>[5x]ARVNAQTGAPDILTSLDEKSVSYDTVMDKYWLSQYVIARETYDWYTLQKDYETVGMLSSPSEGQSYASQFQGD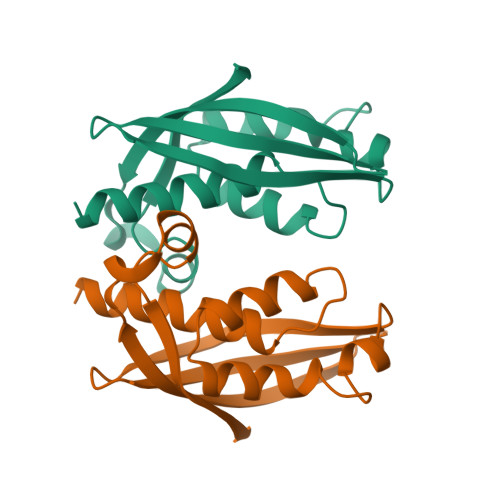KALDKQYGSNVRTSVTIVSIVPNGKGIGTVRFAKTTKRTNETGDGETTHWIATIGYQYVNPSLMSESARLTNPLGFNVTSYRVDPEMGVVQ> SMIEDVSLPSQVLQDQRLKELNQQLQDQLAQQTPYQNTKPLQDFKHLVVEESPCVTVKEISLIPLIGQSESDLQQFNFVIKAIKKHPQNILGKCIGTQSLHNIVNYAQNELLKKGFITSQIVVSPQDLNHGNLNLSIQIGRLNKIVIQEGKISSLQLKTGLPFKAGDIVNLKRLDQGLENLKRVYAVDMQITPATAQDKELTGYSDLILKLQALQKVNFNLSVDDSGNQDTGTYMGNIGIGINNPFHLNDILSLNVSHSLDDFHESLNRSYFISYQLPVGYYDL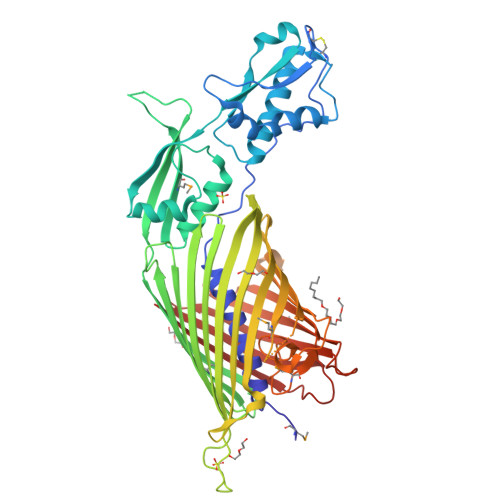GFSYNDYQYRQGTVAPESGYPVIYHGNSQQANLNLSRVISRSGQHKTSVYGKLYHKESQSFLNDIEINVLHRKTSGWNLGVQHRQYLGNAVLDGSIDYRRGMGVGARTAPEENITDVYGNHLPVEGYSRAPLWSADLRYTTPFLLLDKPAQYRLNWRGQYAPKILVPNDRFYIGGRYSVRGFDGELMLSGDNGQYVQQEISLNAPIPNTQFYMAVDQGWVNGRNSIPGQRYLLGSVLGLRTYQNSFYLDAFTGRGLIAPDSIKKDWVTGFSINLSY>MNVSQSNSFGFWDGTSTQAEITHSFDHYIGSAFDASNNNVAVTGNVSATLNVLAGDDKVSIDGNVEDVLVAANVAVLDMGTGNDQLYVAGDVLGKIDAGTGNDEIYIKGDVSAAVDAGTGNDEVYIGGNLSGDLDAGTDNDNIQIGGDVNAALNAGTGNDNLIIGHDVSGIVNMGTDNDTVEVGRTINASGKVLLDTGDDSLLVSGDLFGEVDGGTGNDTIIIAGKVSGNIQGGTGNDIV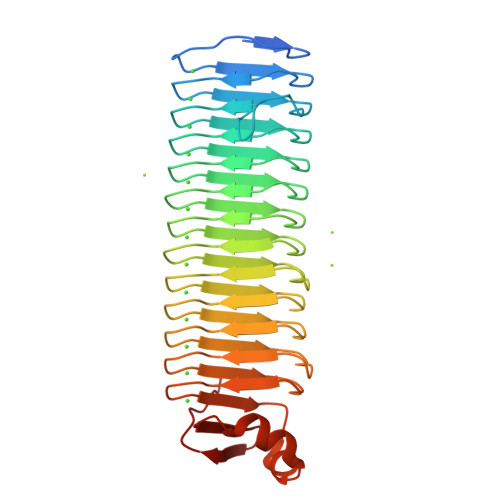RVQSQVWAEANISLGTGDDVLIVEHELHGTVAGNEGDDSIYLKFYTKEQYNNNSDLRNRVANFEHIRVSDGVVKGSPADFADY[4x]>MTLTASSSSRAVTNSPVVVALDYHNRDDALAFVDKIDPRDCRLKVGKEMFTLFGPQFVRELQQRGFDIFLDLKFHDIPNTAAHAVAAAADLGVWMVNVHASGGARMMTAAREALVPFGKDAPLLIAVTVLTSMEASDLVDLGMTLSPADYAERLAALTQKCGLDGVVCSAQEAVRFKQVFGQEFKLVTPGIRPQGSEAGDQRRIMTPEQAL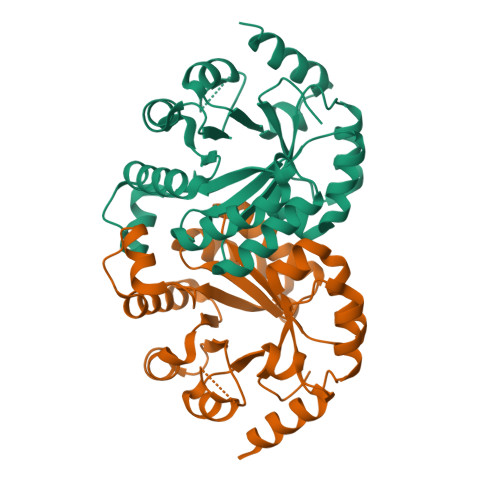SAGVDYMVIGRPVTQSVDPAQTLKAINASLQRSA[2x]The CzcR-CzcS TCS in P. aeruginosa is responsible for numerous cellular processes, including Zn(II) resistance, carbapenem antibiotic resistance, quorum sensing, and virulence regulation. Under direct stimulation by Zn(II), the histidine kinase (HK) CzcS auto-phosphorylates on its conserved histidine residue. In the CzcR-CzcS TCS, the HK CzcS is predicted to be the transmembrane sensor-transmitter, and it contains three functional domains. The stimulus is detected by the periplasmic sensor domain and transmitted across the membrane to the cytoplasmic kinase domain.

Given the pivotal role of the extracellular sensor domain in signal recognition and transduction, we determined the crystal structure of the CzcS sensor domain (CzcS SD) in the presence of Zn(II) (referred as CzcS-Zn hereafter). The structure belongs to the C2 space group and it contains two molecules (CzcS SD, amino acids 40–166 in the CzcS protein) per asymmetric unit. The structure of CzcS SD is a mixed α/β-fold in nature, which can be divided into two domains. The N-terminal helix-loop-helix domain is composed of the H1 α-helix (residues 40–60), the connecting loop (residues 61–66), and the H2 α-helix (residues 67–81). The C-terminal domain contains five β-strands (S1-S5) and one 03B1-helix (H3). In the structure of CzcS-Zn, the N-terminal helix-loop-helix domain is tilted away from the central five anti-parallel β-sheet, which may be caused by the Zn(II) binding at the H1 and H1’ α-helices. Two Zn(II) ions are captured in the structure of CzcS-Zn. In the symmetry operation, this CzcS molecule can form a homodimer, and the Zn(II) is exclusively buried between the central parallel H1 and H1’ α-helices which constitute the dimer interface. A distorted tetrahedral geometry is adopted by Zn(II) to coordinate with the symmetric ligands (His55/Asp60 and His55’/Asp60) from the H1 and H1’ α-helices, respectively. The mutagenesis analyses corroborate the crucial role of the His55 and Asp60 in Zn(II) sensing.

>[2x]GPHMASARERENLQLKLEQIRHSLEDDLDLRSDPAVQAHALQDQLVAHSGLHLSILDSRSGQPLMSFGDQAAASVAANRALLARLQADARQPVFQSWSTGNDQRLLSIGASMRMKNGTPVQVLLSSERNADE>GPLGSDASTKKLSESLKRIGDELDSNMELQRMIAAVDTDSPREVFFRVAADMFSDGNFNWGRVVALFYF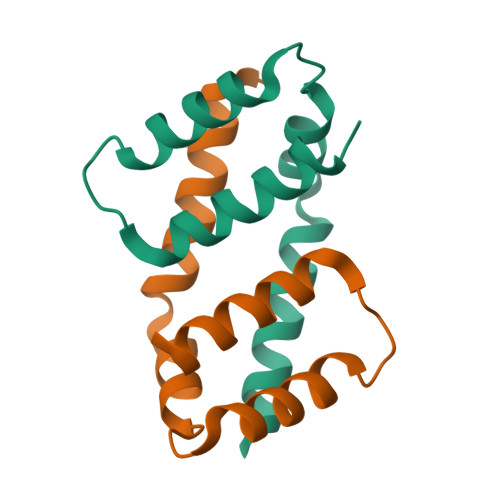ASKLVLKALSTK[8x]> MEEFVN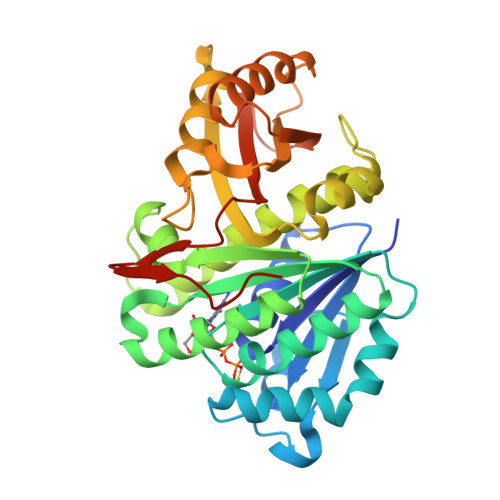PCKIKVIGVGGGGSNAVNRMYEDGIEGVELYAINTDVQHLSTLKVPNKIQIGEKVTRGLGAGAKPEVGEEAALEDIDKIKEILRDTDMVFISAGLGGGTGTGAAPVIAKTAKEMGILTVAVATLPFRFEGPRKMEKALKGLEKLKESSDAYIVIHNDKIKELSNRTLTIKDAFKEVDSVLSKAVRGITSIVVTPAVINVDFADVRTTLEEGGLSIIGMGEGRGDEKADIAVEKAVTSPLLEGNTIEGARRLLVTIWTSEDIPYDIVDEVMERIHSKVHPEAEIIFGAVLEPQEQDFIRVAIVATDFPEEKFQVGEKEVKFKVIKKLHHHHHH> MSQPKPILYYDERSPPVRSCLMLIKLLDIDVELRFVNLFKGEQFQKDFLALNPQHSVPTLVHGDLVLTDSHAILIHLAEKFDEGGSLWPQEHAERMKVLNLLLFECSFLFRRDSDFMSATVRQGFANVDVAHHERKLTEAYIIMERYLENSDFMAGPQLTLADLSIVTTLSTVNLMFPLSQFPRLRRWFTAMQQLD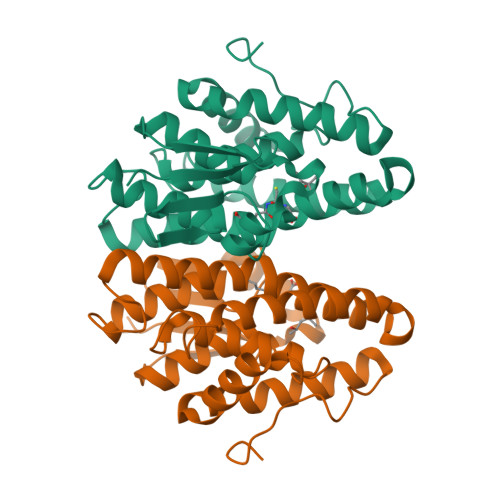AYEANCSGLEKLRQTMESVGSFQFPSSSAVVTEKVEHHHHHH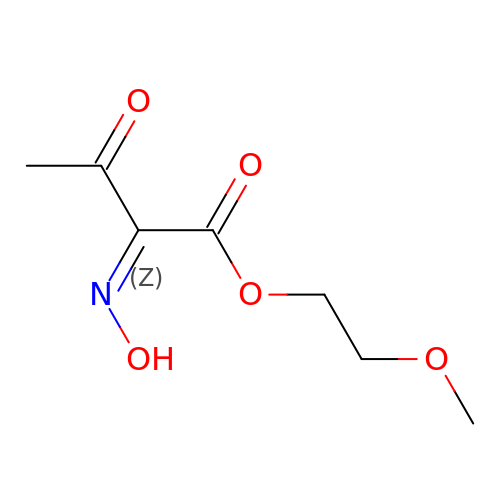2-methoxyethyl (2~{Z})-2-hydroxyimino-3-oxidanylidene-butanoate | C7 H11 N O5 | QNWLIKDDTJMEGE-VURMDHGXSA-N> MGAHASVIKPEMKIKLRMEGAVNGHKFVIEGEGIGKPYEGTQTLDLTVEEGAPLPFSYDILTPAFQWGNRAFTKYPEDIPDYFKQAFPEGYSWERSMTYEDQGICIAT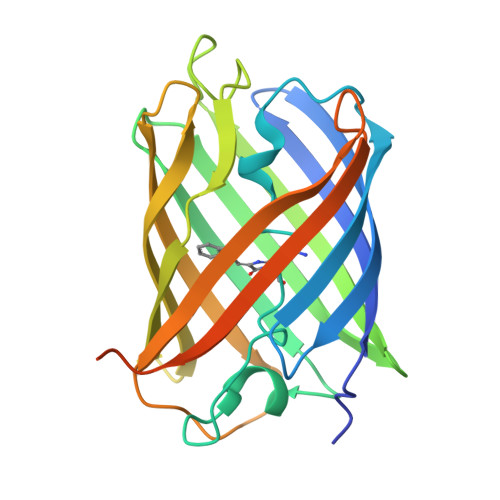SDITMEGDCFFYEIRFDGTNFPPNGPVMQKKTLKLIDATEKMYVEDGVLKGDVEMALLLEGGGHYRCDFKTTYKAKKDVRLPDAHEVDHRTEILSHDKDYNKVRLYEHAEARYSGGGSGGGASGKPIPNPLLGLDSTHHHHHH> MVGLTTLFWLGAIGMLVGTLAFAWAGRDAGSGERRYYVTLVGISGIAAVAYVVMALGVGWVPVAERTVFAPRYINWILTTPLIVYFLGLLAGLDSREFGIVITLNTVVMLAGFAGAMVPGIERYALFGMGAVAFLGLVYYLVGPMTESASQRSSGIKSLYVRLRNLTVILWAIYPFIWLLGPPGVALLTPTVDVALIVYLDLVTKVG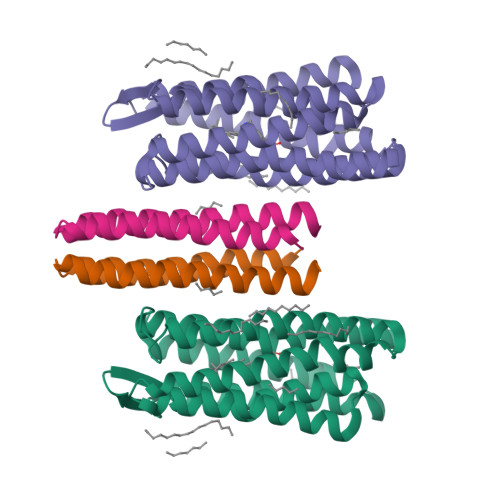FGFIALDAAATLRAEHGESLAGVDTDAPAVADHHHHHH;> MSLNVSRLLLPSRVRHSYTGKMGAVFIFVGALTVLFGAIAYGEVTAAAATGDAAAVQEAAVSAILGLIILLGINLGLVAATLGGDTAASLSTLAAKASRMGDGDLDVELETRREDEIGDLYAAFDEMRQSVRTSL Cysteamine dioxygenase (ADO) plays a vital role in regulating thiol metabolism and preserving oxygen homeostasis in humans by oxidizing the sulfur of cysteamine and N-terminal cysteine-containing proteins to their corresponding sulfinic acids using O2 as a cosubstrate. Among all thiol dioxygenases, ADO stands out for its broader spectrum of substrates. It is the only enzyme of this protein family that oxidizes both small-molecule and protein substrates. Hence, in addition to regulating thiol metabolism, ADO initiates a transduction cascade, signaling hypoxia and preserving oxygen homeostasis in humans. pmcThiol dioxygenases constitute a family of nonheme iron enzymes containing a ferrous iron center coordinated by three histidine residues.

Herein, we report the first crystal structure of human ADO at a resolution of 1.78 Å with a nickel-bound metal center. Crystallization was achieved through both metal substitution and C18S/C239S double mutations. In order to obtain hADO with a homogeneous metal center and prevent oxidation via the iron center, hADO cell culture was grown with minimal media supplemented with NiSO4 during induction of hADO expression. Most of the polypeptide residues are observed except the N-terminal tag, residues 22–40 and 230–239. Despite the flexibility, the core of the hADO structure is a “jelly roll” β-barrel that supports a catalytic center. The structure of hADO shows a metal ion octahedrally coordinated by three histidine residues and three water molecules, which is a typical ligand scaffold for thiol dioxygenases. The protein-derived ligands are His112 and His114 from Loop 3 and His193 from β6. The metal center of ADO sits in a tunnel formed by the β-barrel. Instead, residues 137–144 of Loop 4 intrude into the catalytic center of an adjacent, crystallographic symmetry-related molecule, forming interactions with residues at the active site entrance. Additionally, extra electron density was found in the active site cavity, which was best fitted with a glycerol molecule from the cryoprotectant.

> MPRDNMASLIQRIARQASLTFRGSGGGRGASDRDAASGPEAPMQPGFPENLSKLKSLLTQLRAEDLNIAPRKATLQPLPPNLPPVTYMHIYETDGFSLGVFLLKSGTSIPLHDHPGMHGMLKVLYGTVRISCMDKLDAGGGQRPRALPPEQQFEPPLQPREREAVRPGVLRSRAEYTEASGPCILTPHRDNLHQIDAVEGPAAFLDILAPPYDPDDGRDCHYYRVLEPVRPKEASSSASDLPREVWLLETPQADDFWCEGEPYPGPKVFP> MDTTVPTFSLAELQQGLHQDEFRRCLRDKGLFYLTDCGLTDTELKSAKDIVIDFFEHGSEAEKRAVTSPVPTMRRGFTGLESESTAQITNTGSYSDYSMCYSMGTADNLFPSGDFERIWTQYFDRQYTASRAVAREVLRATGTEPDGGVEAFLDCEPLLRFRYFPQVPEHRSAEEQPLRMAPHYDLSMVTLIQQTPCANGFVSLQAEVGGAFTDLPYRPDAVLVFCGAIATLV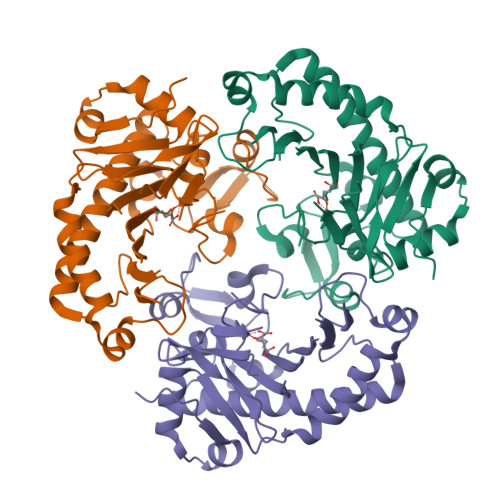TGGQVKAPRHHVAAPRRDQIAGSSRTSSVFFLRPNADFTFSVPLARECGFDVSLDGETATFQDWIGGNYVNIR>MDIDNYRVKPGKRVKLSDWATNDDAGLSKEEGQAQTAKLAGELAEW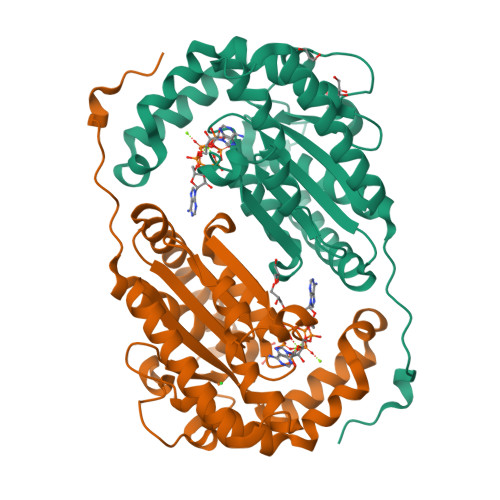QERLYAEGKQSLLLILQARDAAGKDGAVKKVIGAFNPAGVQITSFKQPSAEELSHDFLWRIHQKAPAKGYVGVFNRSQYEDVLVTRVYDMIDDKTAKRRLEHIRHFEELLTDNATRIVKVYLHISPEEQKERLQARLDNPGKHWKFNPGDLKDRSNWDKFNDVYEDALTTSTDDAPWYVVPADRKWYRDLVLSHILLGALKDMNPQFPAIDYDPSKVVIH[2x]>[2x]DAAQPALLQYHYDCGDFGMQLLAYPTRGRTVHFKVLDEFGTRFEVANCSICMHWLNTGEDGGLIFSAGYEGCHVLVKDGRYVLRVQLEEMLLSGVVAASYEVQMTCPRPAGYEILRDEKVHHHHHHHHQRPDRGNS

Vertebrate oocytes are surrounded by a specialised extracellular coat that is referred to as zona pellucida in mammals (ZP) and vitelline envelope in non-mammals (VE). Although their fine morphological appearance differs between classes, all vertebrate egg coats consist of filaments made up of a variable number of glycoprotein components that polymerise using a common ZP module. Accordingly, a recombinant construct corresponding to the predicted ZP-N1 domain of cZP1 (cZP1-N1) is secreted both as a monomeric and a disulphide-bonded dimer, whereas a protein encompassing the trefoil domain and C-terminal ZP module of cZP1 (cZP1L600-R958) does not form intermolecular disulphides. Thus, by recapitulating the oligomeric status of full-length cZP1, cZP1-N1 harbours its cross-linking function.

Examination of the zinc-SAD data used for phasing revealed that asymmetric interaction of the cZP1-N1 homodimer moieties creates a negatively charged pocket where H71(A) coordinates a Zn2+ ion that faces the C269(A)-C390(A) intramolecular disulphide, as well as the C66 cross-link. The anomalous difference map of the data also shows a peak near H71(B) but, consistently with the much lower accessibility of the latter due to crystal packing, this site is weaker than the previous (~6 σ vs. 11 σ). In the Zn2+-soaked crystal, where H71(A) adopts a different orientation and is too far from C390 (A) to make an hydrogen bond, the C269(A)-C390(A) disulphide is partially reduced (most likely due to radiation damage) and H91(A) adopts two alternative conformations, one of which no longer stacks against W72(B) and chelates the Zn2+ together with H71(A) itself. Accordingly, molecular dynamics (MD) simulations suggest that, in solution, the two His residues can stably coordinate a zinc ion together with four water molecules. Taken together, these observations indicate that homodimerisation of hZP1 depends on the same His residues that form a Zn2+-binding site in cZP1-N1. The observation that a Zn2+ ion can be bound by two His residues of cZP1-N1, one of which is invariant (cZP1 H71/hZP1 H82) and the other almost completely conserved (cZP1 H91/hZP1 H102), also raises a possible connection with the zinc spark response of mammalian oocytes to activation. The presence of a conserved Zn2+-binding site in ZP1, together with the finding that mutation of the two Zn2+-binding His severely impairs homodimerisation of hZP1-N1, suggests that zinc ions released by the zygote could modulate the architecture of the ZP by altering the conformation of its ZP1 cross-links.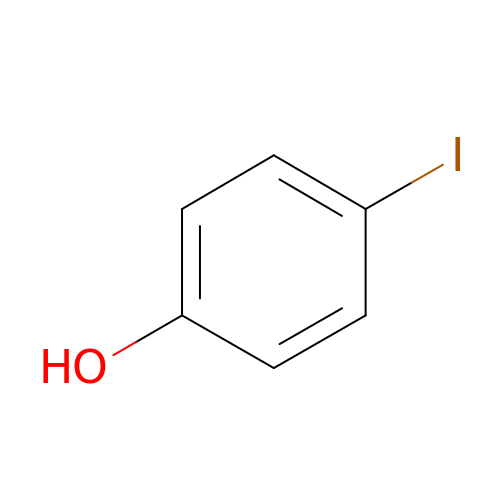4-IODOPHENOL | C6 H5 I O | VSMDINRNYYEDRN-UHFFFAOYSA-N>SNAVGTGGDKAYCVVVDGMGGMIRGDEAAQRALSASVGVLDAGGSPLDAVLAAQAAVHRWASQGGILGRTGATMAVAAVNLRDGTLEWASVGDCRVYLFKGGRLSRLSLDHNVSSEMVLLGRGPVPGPAGEMITSFIGIENLTEISTSE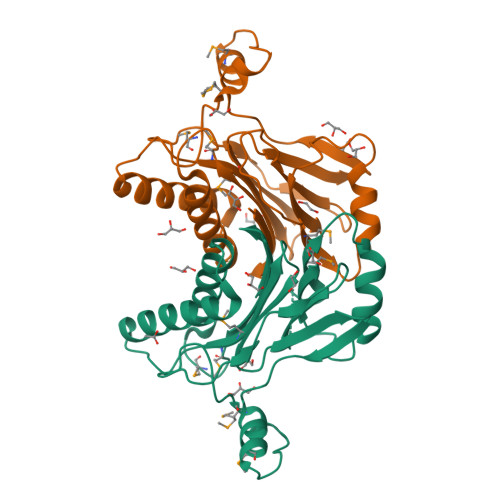APLPLEAGEGVLVVSDGVYRSLHEDRIAMALSRGSDARGILQEVEAQGRPYQDNATLALVIL[2x]>[2x]MSTKSGTN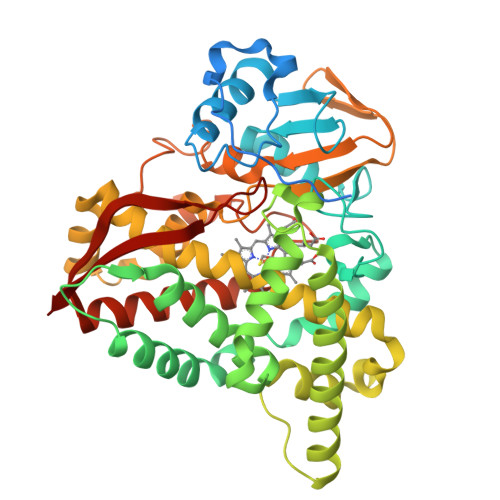DAMQTKMINATSRLVPMHLQIKALKSLMKAKKKALGSTRPQVKFLERPVPDVNTLALEDIDTSNPFLYRQDQWGAYFKRLRDEAPVHFQKSSQFGPFWSVTRYEDILFVDKNHELFSSEPQIILGDPPEGLSVEMFIAMDPPKHDVQRRAVQGVVAPQNLKEMEGLIRQRAAEVLDSLPLDKAFNWVPAVSKELTGRMLATLLDFPYEQRHKLVDWSDRLSGASSATGGEFTDEDIMFDDAADMAWSFSRLWRDKEARRKAGEPPGFDLISMLQSNKDTRDLINRPMEFIGNLALLIVGGNDTTRNSMSGGVLALNQFPEEFIKLKKNPELIPNMVSEIIRWQTPLAHMRRVATQDVELRGQTIKKGDRVLMWYASGNRDERKFENPDQLIIDRKDARNHISFGYGIHRCMGNRLAELQLRILWEELLKRFDNIEVVGEPERVQSNFVRGYSKLMVKLTAKN>ENLYFQGKTVVFVYKDTLKSYKEKFLLKIEKDLKNHHEYYTLKLDDLSEVVEILEENSRICCIVLDRASFNIEAFHNIAHLNTKLPIFVASDYSQSIKLNLRDFNLNINFLQYDALAGEDSDFIHKTITNYFNDILPPLTYELFKYSKSFNSAFCTPGHQGGYGFQRSAVGALFYDFYGENIFKTDLSISMKELGSLLDHSEAHKDAEEYISKVFKSDRSLIVTNGTSTANKIVGMYSVADGDTILVDRNCHKSVTHLMMMVDVNPIYLKPTRNAYGIIGGIPKKEFKRETIQEKIDNSNIADKWPEYAVVTNSTYDGILYNTDTIHRELDVKKLHFDSAWIPYAIFHPIYKHKSAMQIEPRPEHIIFETQSTHKLLAAFSQSSMLHIKGDYNEEVLNEAFMLHTSTSPFYPIVASVETAAAMMEGEQGYNLIDKTINLAIDFRRELIKLRSEANGWFFDVWQPDNISNKEAWLLRNADKWHGFKNVDGDFLSLDPIKITILTPGIKDNDVQDWGVPADVVAKFLDEHDIVVEKSGPYSLLFIFSLGTTKAKSVRLISVLNKFKQMYDENTLVEKMLPTLYAEDPKFYEDMRIQEVSERLHQYMKEANLPNLMYHAFNVLPEQQLNPHRAFQ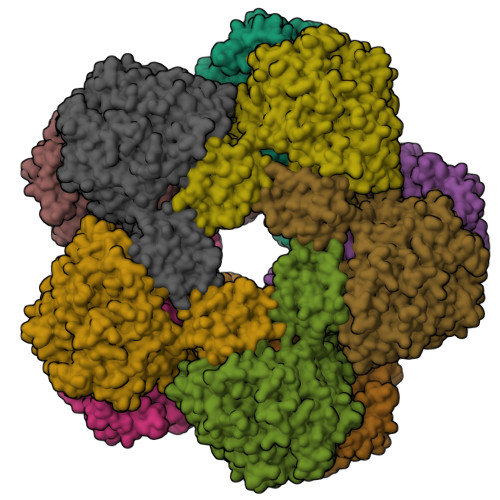KLLKGKVKKVPLAELYEHTSAVMILPYPPGIPVIFPGEKITEESKVILDFLLMLEKIGSMLPGFDTDIHGPERAKDGKLYIKVID[5x]>[2x]YGPKGPKGPKGKPGPDGDPGDPGDPGPKGPKG;>[2x]Y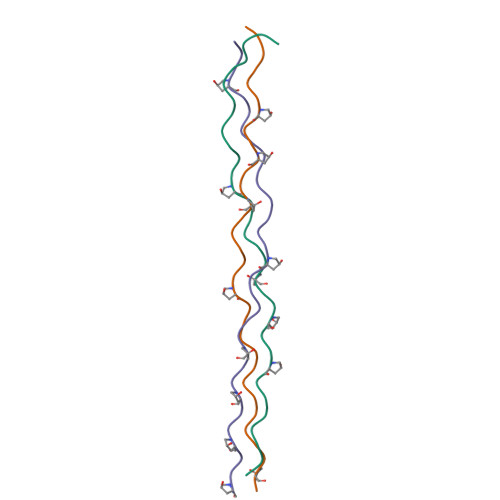GPDGDPGDPGDPGPDGKPGPDGPDGPDGDPG;>[2x]YGKPGPDGPDGPKGKPGPKGKPGKPGKPGKPG N-[(8R)-4-(4-chloro-3-fluorophenyl)-5,6,7,8-tetrahydroisoquinolin-8-yl]propanamide 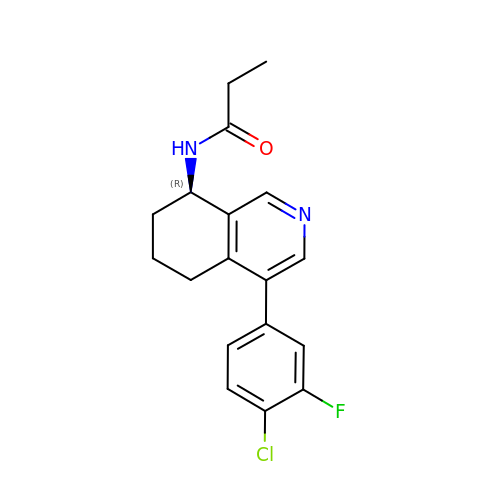| C18 H18 Cl F N2 O | BTXHAHICPWSTRI-QGZVFWFLSA-N>[6x]GHMGLSDLEALRKKIEEVGMPEAVKTKALKELDRLERMQQGSPEATVARTYLDWLTEVPWSKADPEVLDINHTRQVLDEDHYGLKDVKERILEYLAVRQLTQGLDVRNKAPILVLVGPPGVGKTSLGRSIARSMNRKFHRISLGGVRDEAEIRGHRRTYIGAMPGKLIHAMKQVGVINPVILLDQIDKMSSDWRGDPASAMLEVLDPEQNNTFTDHYLDVPYDLSKVFFITTANTLQTIPRPLLDRMEVIEIPGYTNMEKQAIARQYLWPKQVRESGME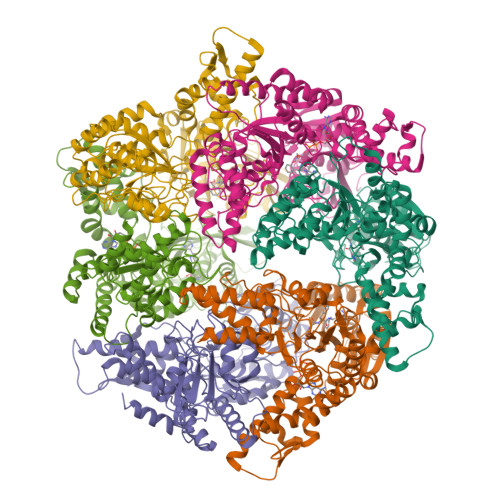GRIEVTDAAILRVISEYTREAGVRGLERELGKIARKGAKFWLEGAWEGLRTIDASDIPTYLGIPRYRPDKAETEPQVGTAQGLAWTPVGGTLLTIEVAAVPGSGKLSLTGQLGEVMKESAQAALTYLRAHTQDYGLPEDFYNKVDLHVHVPDGATPKDGPSAGITMATAIASALSRRPARMDIAMTGEVSLRGKVMPIGGVKEKLLAAHQAGIHKIVLPKDNEAQLEELPKEVLEGLEIKLVEDVGEVLEYLLLPEPTMPPVVQPSDNRQQPGAGA> GAMVNCGHVTAYGPGLTHGVVN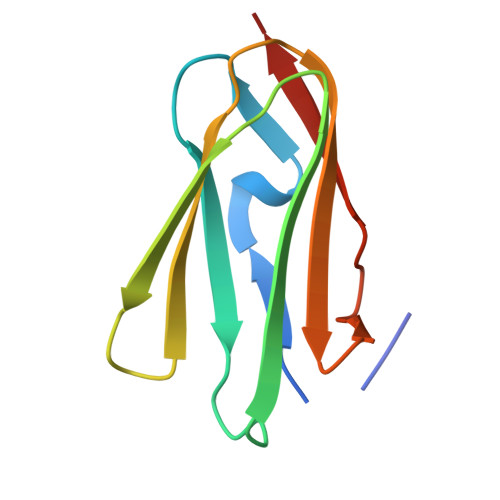KPATFTVNTKDAGEGGLSLAIEGPSKAEISCTDNQDGTCSVSYLPVLPGDYSILVKYNEQHVPGSPFTARVTGDD>[2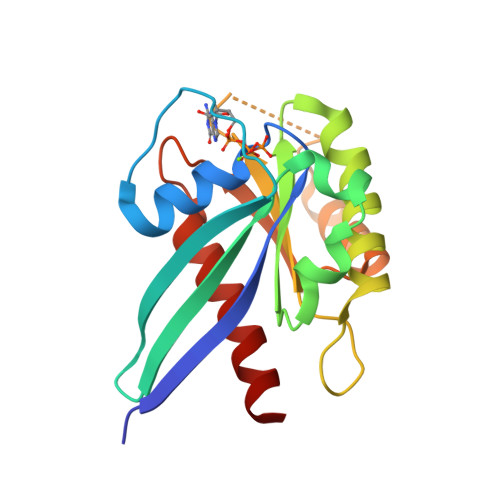x]SMETREHLFKVLVIGELGVGKTSIIKRYVHQLFSQHYRATIGVDFALKVLNWDSRTLVRLQLWDIAGLERFGNMTRVYYKEAVGAFVVFDISRSSTFEAVLKWKSDLDSKVHLPNGSPIPAVLLANKCDQNKDSSQSPSQVDQFCKEHGFAGWFETSAKDNINIEEAARFLVEKILVNHQS> QYSPNTQQGRTSIVHLFEWRWVDIALECERYLAPKGFGGVQVSPPNENVAIYNPFRPWWERYQPVSYKLCTRSGNEDEFRNMVTRCNNVGVRIYVDAVINHMCGNAVSAGTSSTCGSYFNPGSRDFPAVPYSGWDFNDGKCKTGSGDIENYNDATQVRDCRLTGLLDLALEKDYVRSKIAEYMNHLIDIGVAGFRLDASKHMWPGDIKAILDKLHNLNSNWFPAGSKPFIYQEVIDLGGEPIKSSDYFGNGRVTEFKYGAKLGTVIRKWNGEKMSYLKNWGEGW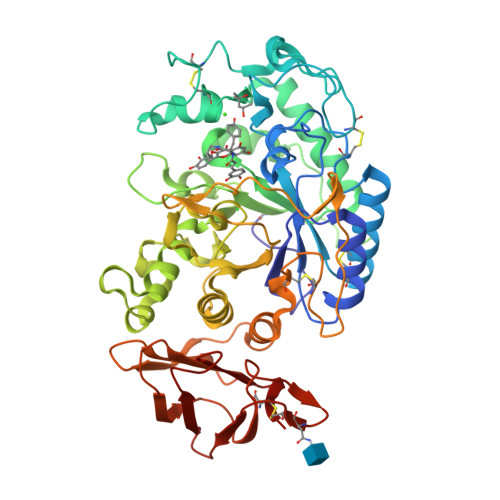GFVPSDRALVFVDNHDNQRGHGAGGASILTFWDARLYKMAVGFMLAHPYGFTRVMSSYRWPRQFQNGNDVNDWVGPPNNNGVIKEVTINPDTTCGNDWVCEHRWRQIRNMVIFRNVVDGQPFTNWYDNGSNQVAFGRGNRGFIVFNNDDWSFSLTLQTGLPAGTYCDVISGDKINGNCTGIKIYVSDDGKAHFSISNSAEDPFIAIHAESKL>[5x]GQDMVSPPPPIADEPLTVNTGIYLIECYSLDDKAETFKVNAFLSLSWKDRRLAFDPVRSGVRVKTYEPEAIWIPEIRFVNVENARDADVVDISVSPDGTVQYLERFSARVLSPLDFRRYPFDSQTLHIYLIVRSVDTRNIVLAVDLEKVGKNDDVFLTGWDIESFTAVVKPANFALEDRLESKLDYQLRISRQYFSYIPNIILPWLFILFI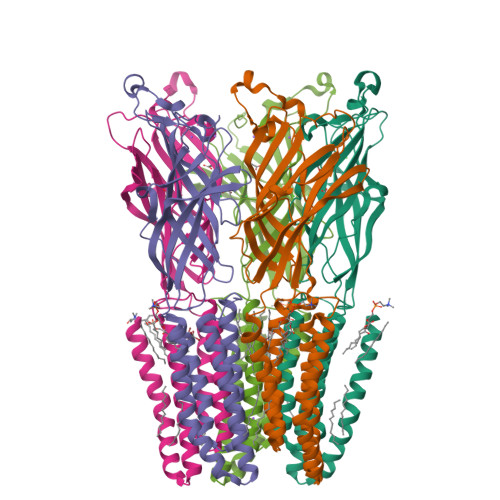SWTAFWSTSYEANVTLVVSTLIAHIAFNILVETNLPKTPYMTYTGAIIFMIYLFYFVAVIEVTVQHYLKVESQPARAASITRASRIAFPVVFLLANIILAFLFFGFGYPYDVPDYA> VVGGEDAKPGQFPWQVVLNGKVDAFCGGSIVNEKWIVTAAHCVETGVKITVVAGEHNIEETEHTEQKRNVIRIIPHHNFNAAINTYNHDIALLELDEPLVLNSYVTPICIADKEYTNIFLKFGSGYVSGWGRVFHKGRSALVLQYLRVPL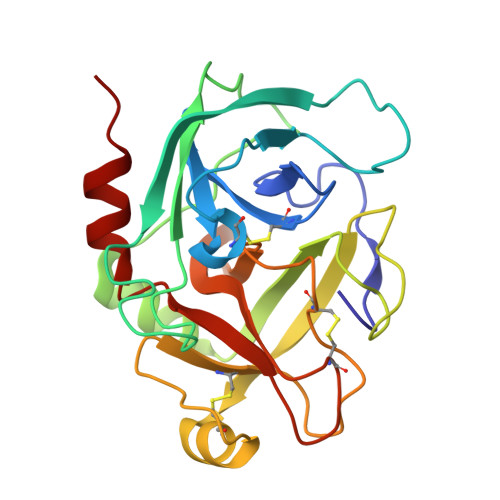VDRATCLRSTKFTITNNMFCAGFHEGGRDSCQGDSGGPHVTEVEGTSFLTGIISWGEECAMKGKYGIYTKVSRYVNWIKEKTKLT>RFLKVKNWETDVVLTDTLHLKSTLETGCTEHICMGSIVLPSQHTRKPEDVRTKDQLFPLAKEFLDQYYSSIKRFGSKAHMDRLEEVNKEIESTSTYQLKDTELIYGAKHAWRNASRCVGRIQWSKLQVFDARDCTTAHGMFNYICNHVKYATNKGNLRSAITIFPQRTDGKHDFRVWNSQLIRYAGYKQPDGSTLGDPANVQFTEICIQQGWKAPRGRFDVLPLLLQANGNDPELFQIPPELVLEVPIRHPKFDWFKDLGLKWYGLPAVSNMLLEIGGLEFSACPFSGWYMGTEIGVRNYCDNSRYNILEEVAKKMDLDMRKTSSLWKDQALVEINIAVLYSFQSDKVTIVDHHSATESFIKHMENEYRCRGGCPADWVWIVPPMSGSITPVFHQEMLNY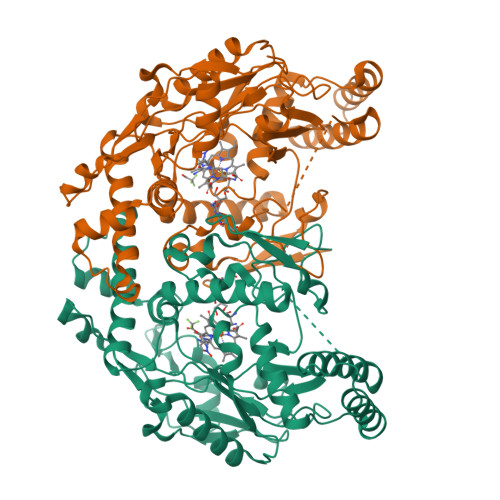RLTPSFEYQPDPWNTHVWKG[2x]Here, we presented the X-ray structures of dimeric KillerOrange and monomeric mKillerOrange, the only known to date GFP-photosensitizers with Trp-based chromophore. To further expand the toolkit of available phototoxic proteins we have very recently come up with a blue-shifted KillerRed variant carrying tryptophan-based chromophore (substitutions: Gly3Cys, Tyr66Trp, Asp113Ser, Asn145Ser, Phe177Leu, Tyr221His, Glu236Gln) named KillerOrange. We also constructed monomeric mKillerOrange by introduction of the single Tyr66Trp substitution in SuperNova, a monomeric variant of KillerRed. The principal structural fold of the monomer in KillerOrange/mKillerOrange, shared with all members of the GFP family, is an 11-stranded β-barrel having loops from both sides and the chromophore (matured from Gln65-Trp66-Gly67 sequence) embedded in the middle of the internal α-helix wound around the β-barrel axis.

The crystal asymmetric unit of KillerOrange contains two dimers and one monomer forming a dimer with the symmetry related subunit, while the crystal asymmetric unit of mKillerOrange contains one monomer. The dimeric structure of KillerOrange comprises two monomers related by a non-crystallographic 2-fold symmetry axis that are positioned at an angle of ~120° relative to each other. The contact area (~1400 Å2 per monomer) between the subunits is stabilized by symmetry related van der Waals contacts, two weak hydrogen bonds between the side chain of His148 (A/D) and the carbonyl of Glu146 (D/A), and two strong peripheral salt bridges between Glu99 (A/D) and Arg158 (D/A). Two aromatic side chains of Phe162 from each subunit make a stabilizing stack (at ~3.6 Å) shielded by side chains of four nearest His148/176 (A/D) and two Leu160 (D/A) residues at the interface center near the symmetry axis. In KillerOrange dimer, the irregular C-terminal tail (residues 224–230) sticks to the surface of the interacting subunits, contributing to the interface stabilization. The contact surface between the monomers of the adjacent dimers is smaller (~735 Å2 per monomer) than within a dimer and is stabilized by two salt bridges, two hydrogen bonds, and a few hydrophobic contacts. A continuous chain of seven hydrogen-bonded water molecules in the channel covers the distance of ~20 Å from catalytic Glu218 in the chromophore area to Pro192 at the bottom of β-barrel. The side chain of Trp66 of the chromophore in KillerOrange and mKillerOrange adopts an unusual trans-cis conformation, not seen for other Trp-based chromophores before. Ile199Lys replacement in KillerOrange resulted in ~25 nm blue shift of absorption band maxima accompanied by significant decrease of the protein phototoxicity and raise of cyan emission, presumably due to isomerization of Trp66 from dominant trans-cis to minor cis-cis conformation.

>[5x]MRGSHHHHHHGSECGPALFQSDMTFKIFIDGEVNGQKFTIVADGSSKFPHGDFNVHAVCETGKLPMSWKPICHLIQWGEPFFARYPDGISHFAQECFPEGLSIDRTVRFENDGTMTSHHTYELSDTCVVSRITVNCDGFQPDGPIMRDQLVDILPSETHMFPHGPNAVRQLAFIGFTTADGGLMMGHLDSKMTFNGSRAIEIPGPHFVTIITKQMRDTSDKRDHVCQREVAHAHSVPRITSAIGSDQD> QETQGQAAARAAAADLAAGQDDEPRILEAPAPDARRVYVNDPAHF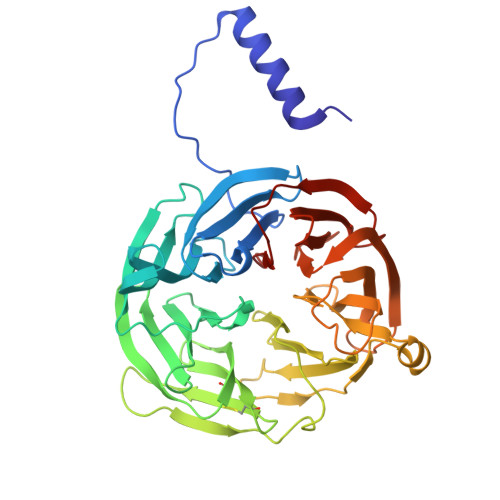AAVTQQFVIDGEAGRVIGMIDGGFLPNPVVADDGSFIAHASTVFSRIARGERTDYVEVFDPVTLLPTADIELPDAPRFLVGTYPWMTSLTPDGKTLLFYQFSPAPAVGVVDLEGKAFKRMLDVPDCYHIFPTAPDTFFMHCRDGSLAKVAFGTEGTPEITHTEVFHPEDEFLINHPAYSQKAGRLVWPTYTGKIHQIDLSSGDAKFLPAVEALTEAERADGWRPGGWQQVAYHRALDRIYLLVDQRDEWRHKTASRFVVVLDAKTGERLAKFEMGHEIDSINVSQDEKPLLYALSTGDKTLYIHDAESGEELRSVNQLGHGPQVITTADMG>QDMEGNGPAAVHYQPASPPRDACVYSSCYSEENVWKLCEYIKNHDQYPLEECYAVFISNERKMIPIWKQQARPGDGPVIWDYHVVLLHVSSGGQSFIYDLDTVLPFPCLFDTYVEDAIKSDDDIHPQFRRKFRVICADSYLKNFASDRSHMKDSSGN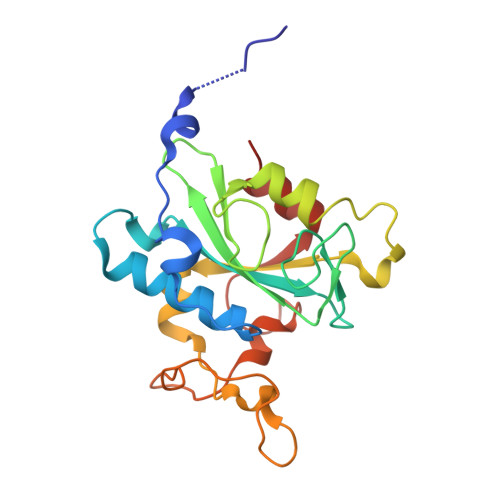WREPPPPYPCIETGDSKMNLNDFISMDPKVGWGAVYTLSEFTHRFGS[2x]> VFPSSVFVPDEWEVSREKITLLRELGQGSFGMVYEGNARDIIKGEAETRVAVKTVNESASLRERIEFLNEASVMKGFTCHHVVRLLGVVSKGQPT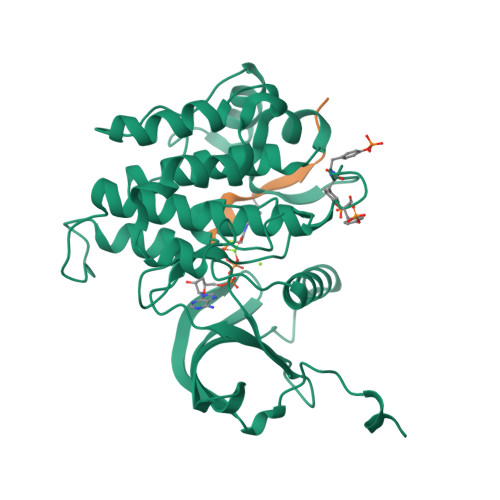LVVMELMAHGDLKSYLRSLRPEAENNPGRPPPTLQEMIQMAAEIADGMAYLNAKKFVHRDLAARNCMVAHDFTVKIGDFGMTRDIYETDYYRKGGKGLLPVRWMAPESLKDGVFTTSSDMWSFGVVLWEITSLAEQPYQGLSNEQVLKFVMDGGYLDQPDNCPERVTDLMRMCWQFNPKMRPTFLEIVNLLKDDLHPSFPEVSFFHSEENK;> PATGDFMNMSPVG> CCUGAGUUCAAUUCUAGCG

The yeast TREX2 complex functions to integrate the nuclear components of the gene-expression pathway with mRNA nuclear export as well as localizing actively expressing genes such as GAL1 to nuclear pores (NPCs). TREX2 is based on a Sac3 scaffold, to which Thp1, Sem1, Cdc31 and two chains of Sus1 bind. Previous work indicated a level of specificity in RNA binding by TREX2 in that polyuridine binds more strongly than other polyribonucleotides, and studies on the human analogue of TREX2 that is based on GANP (the Sac3 homologue) also showed some specificity in binding to a subset of transcripts.

Here, we report the 1.25 Å resolution crystal structure of a 20 nt RNA fragment identified as having a higher affinity for TREX2 than polyuridine. There was no clear electron density for adenine 1, which appeared to be disordered owing to its being displaced to facilitate the canonical C–G pairings between bases 19 and 20 in consecutive duplexes along the crystallographic 31 axis. Consistent with this interpretation, the electron density for the ribose of cytosine 2 was also weak. Although the RNA formed a duplex in the crystals, it appeared to be monomeric in solution and probably formed a hairpin using base pairing analogous to that observed in the duplex. The formation of duplexes from hairpins is favoured at the high ionic strength and RNA concentrations employed for crystallization. A similar amino–imino hydrogen bonding was observed in the Hepatitis C virus internal ribosome entry site eIF3-binding site and thymidylate synthase mRNA, where multiple conformations of this base were also observed.Flavivirus envelope (E) and precursor M (prM) proteins, when ectopically expressed, assemble into empty, virus-like particles (VLPs). Cleavage of prM to M and loss of the pr fragment converts the VLPs from immature to mature particles, mimicking a similar maturation of authentic virions. The icosahedrally symmetric, immature particles contain 180 envelope (E) subunits associated with the same number of membrane-protein precursor (prM) subunits and internal, core (C) protein subunits. Both E and prM are glycoproteins with C-terminal, transmembrane anchors. We describe here the cryo-EM structure of immature, small VLPs (smVLPs) from dengue virus type 2 and show that they have octahedral rather than icosahedral symmetry.

Focused classification and refinement of a symmetry-expanded particle image stack yielded an improved map of the asymmetric unit (three prM-E heterodimers) at 4.3 Å resolution. The asymmetric unit of the octahedral particle is an asymmetric trimer of prM-E heterodimers, just as it is on icosahedral immature virions; the full, octahedrally symmetric particle thus has 24 such asymmetric trimers or 72 prM-E heterodimers in all. We obtained an AlphaFold 2 structure from the DENV2 prM-E sequence, docked three models of the prM-E heterodimer independently into the three subunits of the asymmetric unit, and manually modeled the linker sequence between pr and M. The model was fit to the locally focused map by domain-wise rigid-body fitting, structure morphing, and real space refinement. The stem and transmembrane segments of E and prM were reasonably well defined in the map, in particular for two of the three protomers. Our map is consistent with the revised prM connectivity seen clearly in the structures of immature BinJV and TBEV in which the three pr domains at the tips of an asymmetric threefold cluster connect directly to the three stem and transmembrane anchors (stem-TMs) clustered around the same pseudo-threefold. In our locally refined map, essentially continuous density (weak from residues 215–224, but unambiguously traced for two of the chains and suggested by very weak density for the third) connects each “pr” domain associated with a fusion-loop tip of E with a corresponding stem-TM. One local difference is in the orientation of the prM stem-TM associated with the E subunit marked B in Fig. 3B. In our octahedral smVLP structure, the segment that connects the pr domain and stem-TM of the prM in question allows the B-subunit stem-TM to form an approximately twofold symmetric contact with the stem-TM of prM associated with subunit C—that is, to orient the stem-TM about 180° from its orientation in the full particle. Moreover, this contact is essentially the same as the twofold contact between M proteins in the mature icosahedral particle.

>MRCIGISNRDFVEGVSGGSWVDIVLEHGSCVTTMAKNKPTLDFELIKTEAKQPATLRKYCIEAKLTNTTTDSRCPTQGEPSLNEEQDKRFVCKHSMVDRGWGNGCGLFGKGGIVTCAMFTCKKNMKGKVVQPENLEYTIVITPHSGEEHAVGNDTGKHGKEIKITPQSSITEAELTGYGTVTMECSPRTGLDFNEMVLLQMENKAWLVHRQWFLDLPLPWLPGADTQGSNWIQKETLVTFKNPHAKKQDVVVLGSQEGAMHTALTGATEIQMSSGNLLFTGHLKCRLRMDKLQLKGMSYSMCTGKFKVVKEIAETQHGTIVIRVQYEGDGSPCKIPFEIMDLEKRHVLGRLITVNPIVTEKDSPVNIEAEPPFGDSYIIIGVEPGQLKLNWFKKGSSIGQMIETTMRGAKRMAILGDTAWDFGSLGGVFTSIGKALHQVFGAIYGAAFSGVSWIMKILIGVIITWIGMNSRSTSLSVSLVLVGVVTLYLGVMVQA[3x];>[3x]FHLTTRNGEPHMIVSRQEKGKSLLFKTEDGVNMCTLMAMDLGELCEDTITYKCPFLKQNEPEDIDCWCNSTSTWVTYGTCTTTGEHRREKRSVALVPHVGMGLETRTETWMSSEGAWKHAQRIETWILRHPGFTIMAAILAYTIGTTHFQRALIFILLTAVAPSMT>[2x]SVDLIGINVAGAEFTGGKLPGKHGTHYFFPPEGYFEYWSEQGIHTVRFPLKWERLQPSLNAELDDVYASLVDDMLDQAKENDIKVILDVHNYARYRKKVIGTEDVPVSAYQDLMERIAKRWQGHDALFAYDIMNAPYGSADKLWPAAAQAGIDGVRKYDKKRPLLIEGASWSSAARWPRYADELLKLKDPADNMVFSAHVYIDEDASGSYKKGPGKDFEPMIGVKR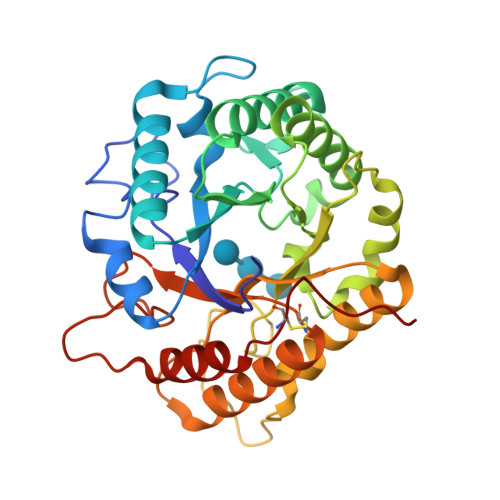VEPFVNWLKEHGKKGHIGEFGIPNDDERWLDAMDKLLAYLNENCIPINYWAAGPSWGNYKLSIEPKDGEKRPQVALLKKYAAKDNCSDFGPAKAE(3Z)-4-{[(4-AMINO-2-METHYLPYRIMIDIN-5-YL)METHYL]AMINO}-3-MERCAPTOPENT-3-EN-1-YL 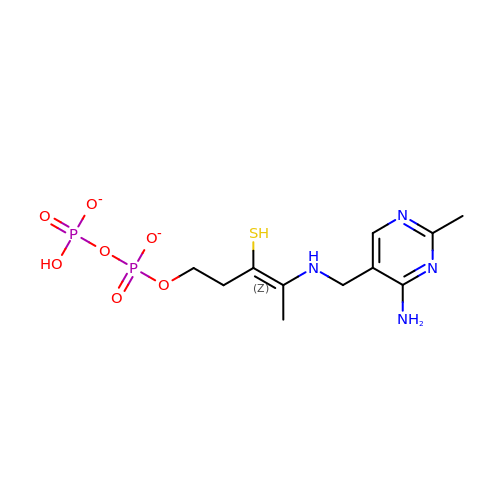TRIHYDROGEN DIPHOSPHATE | C11 H18 N4 O7 P2 S | WTQDUFKDQLXDPH-YFHOEESVSA-L>MAHHHHHHVGTFENITAAPADPILGLADLFRADERPGKINLGIGVYFDETGKCPVLTSVKKAEQYLLENETTKSYLGIDGIPEFGRCTQELLFGKGSALINDKRARTAQTPGGTGALRVAADFLAKNTSVKRVWVSNPSWPNHKSVFNSAGLEVREYAYYDAENHTLDFDALINSLNEAQAGDVVLFHGCCHNPTGIDPTLEQWQTLAQLSVEKGWLPLFDFAYQGFARGLEEDAEGLRAFAAMHKELIVASSYSKNFGLYNERVGACTLVAADSETVDRAFSQMKAAIRANYS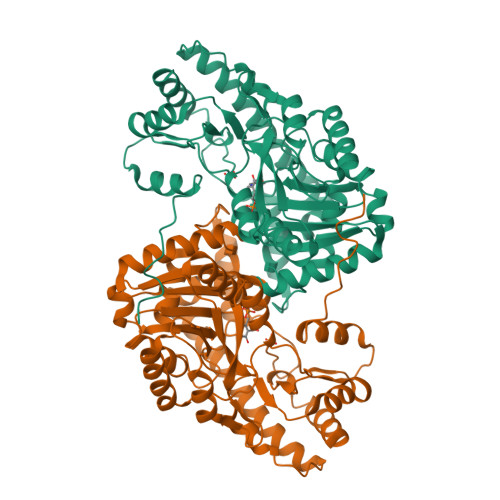NPPAHGASVVATILSNDALRAIWEQELTDMRQRIQRMRQLFVNTLQEKGANRDFSFIIKQNGMFSFSGLTKEQVLRLREEFGVYAVASGRVNVAGMTPDNMAPLCEAIVAVL[2x]> ATLKDITRRLKSIKNIQKITKSMKMVAAAKYARAERELKPARVYGVGSLALYEKADIKTPEDKKKHLIIGVSSDRGLCGAIHSSVAKQMKSEAANLAAAGKEVKIIGVGDKIRSILHRTHSDQFLVTFKEVGRRPPTFGDASVIALELLNSGYEFDEGSIIFNRFRSVISYKTEEKPIFSLDTISSAESMSIYDDIDADVLRNYQEYSLANIIYYSLKESTTSEQSARMTAMDNASKNASEMIDKLTLTFNRTRQAVITKELIEIISGAAALD;> AEAAAAQAPAAGPGQMSFTFASPTQVFFNSANVRQVDVPTQTGAFGILAAHVPTLQVLRPGLVVVHAEDGTTSKYFVSSGSVTVNADSS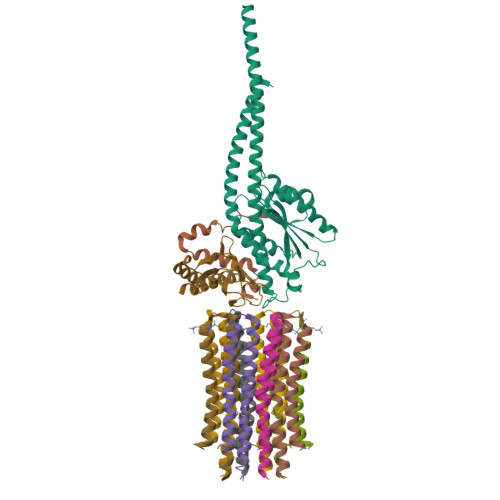VQLLAEEAVTLDMLDLGAAKANLEKAQSELLGAADEATRAEIQIRIEANEALVKALE;> VAYWRQAGLSYIRYSQICAKAVRDALKTEFKANAMKTSGSTIKIVKVKKE;>[8x]DIDTAAKFIGAGAATVGVAGSGAGIGTVFGSLIIGYARNPSLKQQLFSYAILGFALSEAMGLFCLMVAFLILFAM One such mechanism widely found across Firmicute bacteria involves antimicrobial peptide sensing and resistance membrane protein complexes collectively known as Bce modules. These modules are composed minimally of an ATP-binding cassette (ABC) transporter which defends against antimicrobial peptides without transport across the membrane, and an interacting two-component system containing a sensor histidine kinase and response regulator. In this module bceA encodes the ATPase domains, bceB encodes the membrane-spanning permease domain of the ABC transporter BceAB, and bceS encodes the histidine kinase that phosphorylates the response regulator encoded by bceR. Previous studies have established that BceAB mediates resistance against bacitracin, likely by freeing bacitracin from the lipid target undecaprenyl-pyrophosphate (UPP). To understand this critical membrane protein interaction and the molecular details underpinning the Bce module flux-sensing mechanism, we have determined the cryo-EM structure of the complete BceAB-S complex from B. subtilis in nucleotide-free and ATPγS-bound states.

To investigate this hypothesis, we pursued a cryo-EM structure of wild-type BceAB-S with the non-hydrolysable ATP analog ATPγS. Initial 3D classification of the resultant dataset revealed two distinct particle populations, with one population showing a large degree of heterogeneity in the intracellular DHp and CA domains of BceS, and a second population in which the entire BceS kinase was more clearly resolved. Subsequent classification and refinement produced two cryo-EM maps of the ATPγS-bound BceAB-S complex, one of which was obtained at 3.1 Å overall resolution showing high resolution features BceAB and the TM and HAMP domains of BceS, but disordered BceS DHp and CA domains. In both reconstructions the binding of ATPγS induces the BceA nucleotide binding domains (NBDs) to transition from the highly asymmetric configuration observed in the nucleotide-free state, into a conformation that closely resembles that seen in the isolated BceAB transporter bound to ATP. However, close inspection reveals that the BceA subunits are not fully dimerized and ATPγS engages the Walker-A motif and Tyr13 in the A-loop of BceA, but not the signature motif in the opposing BceA monomer. Thus, although ATPγS induced a more symmetrical orientation of BceA monomers within the BceAB-S complex, the monomers are not positioned to support ATP hydrolysis. More importantly, the conformational shifts induced by binding of ATPγS to the BceA subunits do not affect the overall conformation of BceB. Within the ATPγS-bound BceAB-S structure, the BceB TM helix configuration closely resembles that of the nucleotide-free state, rather than the closed conformation seen with isolated BceAB bound to ATP.

> MNINQLILRNLKKNLRNYYLYVFALIFSVALYFAFVTLQYDPAINEVKASIKGAAAIKTASILLVAVVAIFILYANTIFIKRRSKEIGLFQLIGMTKHKIFRILSAENVMLYFGSLAIGVAAGFSISKLVLMILFKIVDVKADAKLHFSEQALVQTVIVFCGIYLLIMIMNYTFIKKQSILSLFKVTSSTEDKVKKISFFQMLIGALGIVLILTGYYVSSELFGGKFKTINELFVAMSFILGSVIIGTFLFYKGSVTFISNIIRKSKGGYLNISEVLSLSSIMFRMKSNALLLTIITTVSALAIGLLSLAYISYYSSEKTAEQNVAADFSFMNEKDAKLFENKLRESNISFVKKATPVLQANVDIANIMDGTPKEMQGDPGNMQLAVVSDKDVKGVDVAAGEAVFSGYTDLLQKIMVFKDSGVIKVKSKHETQPLKYKGLREEFLVSYTFTSGGMPAVIVDDSLFKQLDKDKDPRIQLAQSTFIGVNVKHDDQMEKANELFQQVNKKNEHLSRLDTSAAQKSLFGMVMFIVGFLGLTFLITSGCILYFKQMGESEDEKPSYTILRKLGFTQGDLIKGIRIKQMYNFGIPLVVGLFHSYFAVQSGWFLFGSEVWAPMIMVMVLYTALYSIFGFLSVLYYKKVIKSSL;>[2x]MSGHHHHHHVILEANKIRKSYGNKLNKQEVLKGIDIHIEKGEFVSIMGASGSGKTTLLNVLSSIDQVSHGTIHINGNDMTAMKEKQLAEFRKQHLGFIFQDYNLLDTLTVKENILLPLSITKLSKKEANRKFEEVAKELGIYELRDKYPNEISGGQKQRTSAGRAFIHDPSIIFADEPTGALDSKSASDLLNKLSQLNQKRNATIIMVTHDPVAASYCGRVIFIKDGQMYTQLNKGGQDRQTFFQDIMKTQGVLGGVQHEH;>[2x]MIKAFLIERRSWIAAFLFQQALMLFIAFVDPSISFGNVLYMVYLCILFFIIFLWFRYRKETAFYKSLKTWENNLDVTAINEPETPFEAMVERSIAGQTEHLKQTAARHRLALENEKDELMAWIHEVKTPLTAMHLIIDRMEEKALKSQLSYEWLRIHLLLDQQLHQKRISFIENDLSVEFIQLQPLIFKEIKDLQSWCIQKGIGFDIQLEAKEVLSDAKWLAFIIRQLLTNAVKYSEASEIEIKSFQKGEQTQLQVKDCGRGIDPKDVPRIFDKGFTSTTDHHDQASTGMGLYLAKKAAAPLLIHIDVESEFGAGTVFTLTFPIRNQFEHVISV3-(benzotriazol-1-yl)-5-[1-methyl-5-(1-phenylcyclopropyl)-1,2,4-triazol-3-yl]pyrazin-2-amine 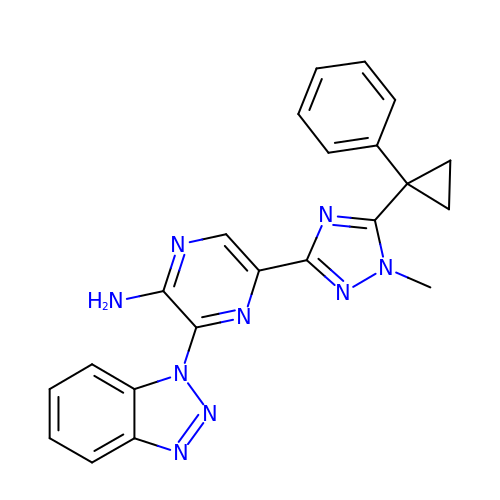| C22 H19 N9 | XOIZTLBSABIUDC-UHFFFAOYSA-N>MENQEKASIAGHMFDVVVIGGGISGLSAAKLLTEYGVSVLVLEARDRVGGRTYTIRNEHVDYVDVGGAYVGPTQNRILRLSKELGIETYKVNVSERLVQYVKGKTYPFRGAFPPVWNPIAYLDYNNLWRTIDNMGKEIPTDAPWEAQHADKWDKMTMKELIDKICWTKTARRFAYLFVNINVTSEPHEVSALWFLWYVKQCGGTTRIFSVTNGGQERKFVGGSGQVSERIMDLLGDQVKLNHPVTHVDQSSDNIIIETLNHEHYECKYVINAIPPTLTAKIHFRPELPAERNQLIQRLPMGAVIKC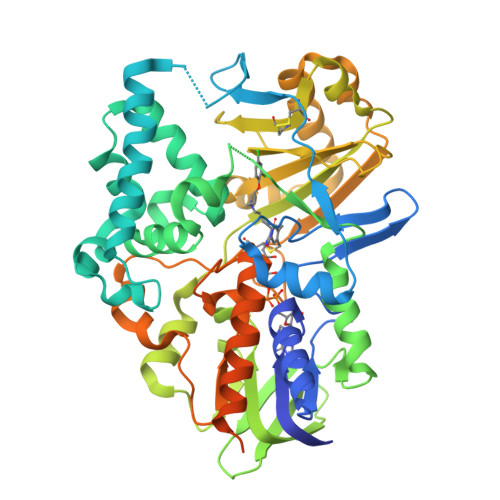MMYYKEAFWKKKDYCGCMIIEDEDAPISITLDDTKPDGSLPAIMGFILARKADRLAKLHKEIRKKKICELYAKVLGSQEALHPVHYEEKNWCEEQYSGGCYTAYFPPGIMTQYGRVIRQPVGRIFFAGTETATKWSGYMEGAVEAGERAAREVLNGLGKVTEKDIWVQEPESKDVPAVEITHTFWERNLPSVSGLLKIIGFSTSVTALGFVLYKYKLLPRS[2x]> MDVLYSLSKTLKDARDKIVEGTLYSNVSDLIQQFNQMIITMNGNEFQTGGIGNLPIRNWNFDFGLLGTTLLNLDANYVETARNTIDYFVDFVDNVCMDEMVRESQRNGIAPQSDSLRKLSGLKFKRINFDNSSEYIENWNLQNRRQ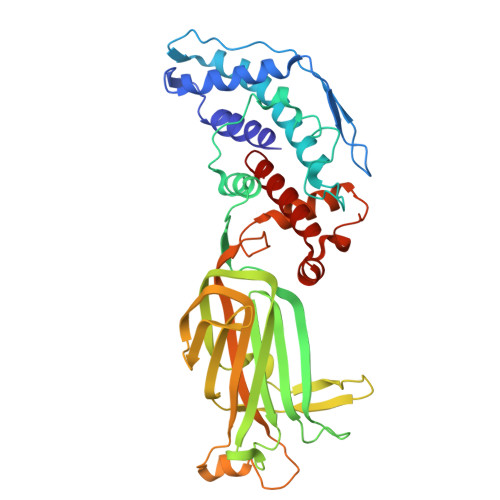RTGFTFHKPNIFPYSASFTLNRSQPAHDNLMGTMWLNAGSEIQVAGFDYSCAINAPANTQQFEHIVQLRRVLTTATITLLPDAERFSFPRVINSADGATTWYFNPVILRPNNVEVEFLLNGQIINTYQARFGTIIARNFDTIRLSFQLMRPPNMTPAVAALFPNAQPFEHHATVGLTLRIESAVCESVLADASETMLANVTSVRQEYAIPVGPVFPPGMNWTDLITNYSPSREDNLQRVFTVASIRSMLVK2-[4-(DIMETHYLAMINO)PHENYL]-6-HYDROXY-3-METHYL-1,3-BENZOTHIAZOL-3-IUM 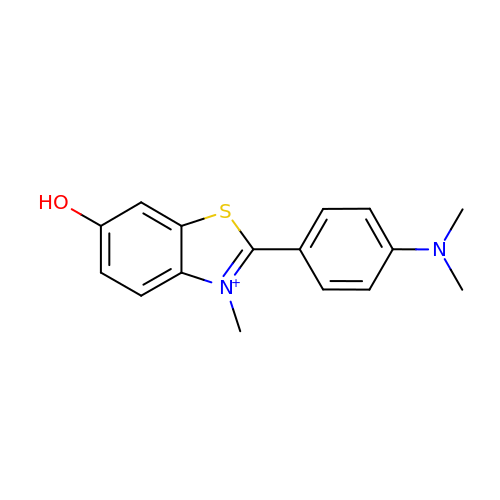| C16 H17 N2 O S | NOVJJPLRUMZSDK-UHFFFAOYSA-O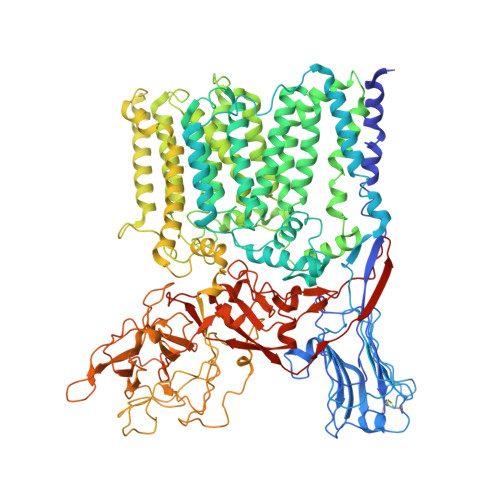> MSGNMDEAVSGNMDEAVSAGKDVRIARWVATIAGLLGFVLSVSIPLLPVTQTTATLNWPQQGRLDNVTAPLISQAPLELTATVPCSVVRDLPPEGGLVFGTAPAEGRDAALNAMLVNVTETRVDVIVRNVVVASVNRDRVAGPDCQRIEITSNLDGTYADFVGLTQISGEDAGKLQRTGYPDPNLRPAIVGVFTDLTGPAPQGLSVSAEIDTRFTTHPTALKLAAMLLAIVSTVIALLALWRLDRLDGRRMHRLIPTRWRTVTAVDGVVVGGMAIWYVIGANSSDDGYILQMARTAEHAGYMANYFRWFGSPEDPFGWYYNVLALMTKVSDASIWIRLPDLICALICWLLLSREVLPRLGPAVAGSRAAMWAAGLVLLGAWMPFNNGLRPEGQIATGALITYVLIERAVTSGRLTPAALAITTAAFTLGIQPTGLIAVAALLAGGRPILRIVMRRRRLVGTWPLIAPLLAAGTVILAVVFADQTIATVLEATRIRTAIGPSQEWWTENLRYYYLILPTTDGAISRRVAFVFTAMCLFPSLFMMLRRKHIAGVARGPAWRLMGIIFATMFFLMFTPTKWIHHFGLFAAVGGAMAALATVLVSPTVLRSARNRMAFLSLVLFVLAFCFASTNGWWYVSNFGAPFNNSVPKVGGVQISAIFFALSAIAALWAFWLHLTRRTESRVVDRLTAAPIPVAAGFMVVVMMASMAIGVVRQYPTYSNGWANIRAFAGGCGLADDVLVEPDSNAGFLTPLPGAYGPLGPLGGEDPQGFSPDGVPDRIIAEAIRLNNPQPGTDYDWNRPIKLDEPGINGSTVPLPYGLDPKRVPVAGTYSTEAQQESRLSSAWYELPARDETERAAHPLVVITAAGTITGESVANGLTTGQTVDLEYATRGPDGTLVPAGRVTPYDVGPTPSWRNLRYPRSEIPDDAVAVRVVAEDLSLSQGDWIAVTPPRVPELQSVQEYVGSDQPVLMDWAVGLAFPCQQPMLHANGVTEVPKFRISPDYYAKLQSTDTWQDGINGGLLGITDLLLRASVMSTYLSQDWGQDWGSLRKFDTVVEATPAELDFGSQTHSGLYSPGPLRIRPHLGGIKAFHHHHHHHHHH>[2x]MSNKYRVRKNVLHLTDTEKRDFVRTVLILKEKGIYDRYIAWHGAAGKFHTPPGSDRNAAHMSSAFLPWHREYLLRFERDLQSINPEVTLPYWEWETDAQMQDPSQSQIWSADFMGGNGNPIKDFIVDTGPFAAGRWTTIDEQGNPSGGLKRNFGATKEAPTLPTRDDVLNALKITQYDTPPWDMTSQN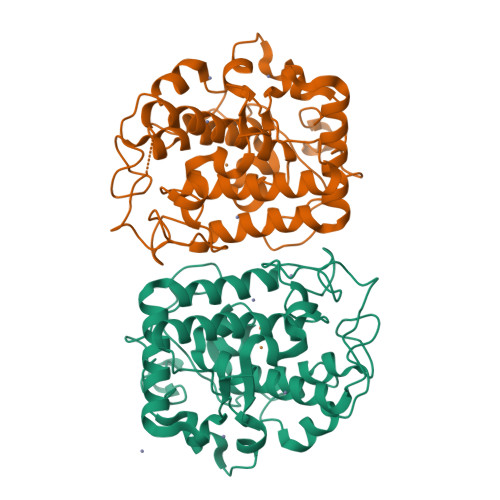SFRNQLEGFINGPQLHNRVHHWVGGQMGVVPTAPNDPVFFLHHANVDRIWAVWQIIHRNQNYQPMKNGPFGQNFRDPMYPWNTTPEDVMNHRKLGYVYDIELRKSKRSSHHHHHH1-({[(1R,2S,3R,5Z,7E,14beta,17alpha)-1,3,25-trihydroxy-9,10-secocholesta-5,7,10-trien-2-yl]oxy}methyl)cyclopropanecarbonitrile | C32 H49 N O4 | 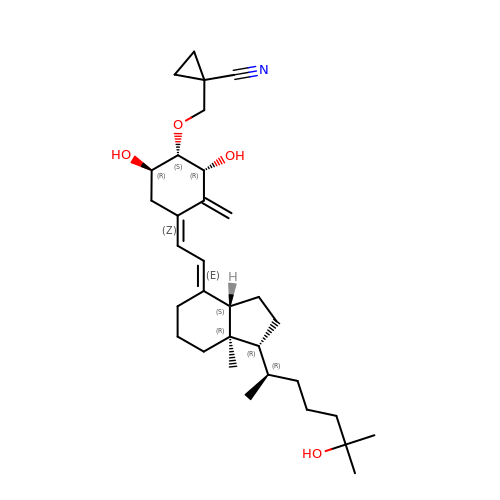XRVHRGHHDVJYGR-IPBGMLIISA-N>[3x]ACDLPCGVYDPAQARIEAESVKAVQEKMAGNDDPHFQTRATVIKEQRAELAKHHVSVL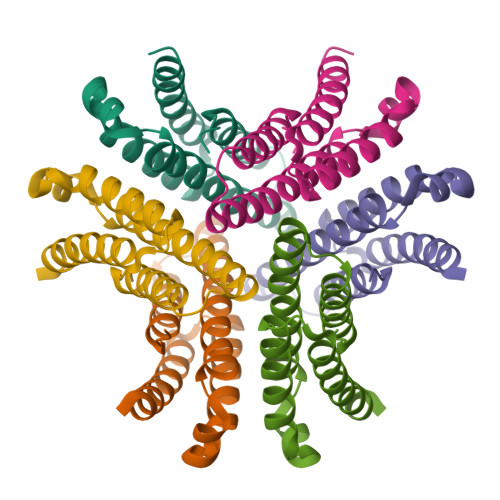WSDYFKPPHFEKYPELHQLVNDTLKALSAAKGSKDPATGQKALDYIAQIDKIFWETKKA>[4x]MTTLTRADWEARAKDLKIEGRA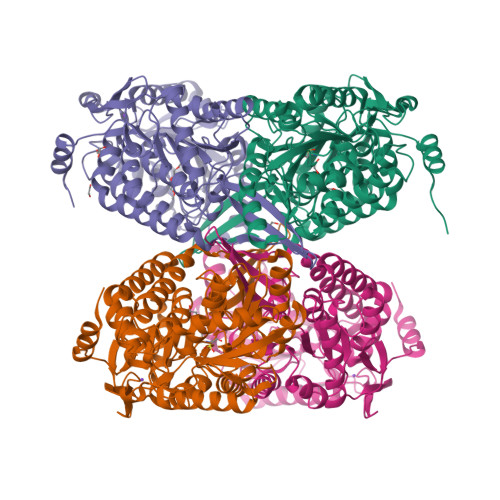FVNGEYSNAASGETFDCLSPVDGRFLAKVASCDLADAEQAVKVARNAFDSGAWSRLAPAKRKQTMIRFADLLLENAEELALLETLDMGKPISDSLHIDVASAANSLRWSAEAIDKIYDEVAATPHAELGLVTREPVGVVAAIVPWNFPLLMSCWKLGPALATGNSVILKPSEKSPLTAIRIAQLAVEAGIPKGVFNVLPGYGHTVGKALALHMDVDTLVFTGSTKIAKQLMVYAGESNMKRVWLEAGGKSPNIVFADAPDLKAAAEAAAGAIAFNQGEVCTAGSRLLVERSIKDKFLPLVIEALKGWKPGNPLDPETNVGALVDTQQMNTVLSYIEAGHNDGAKLVAGGKRTLEETGGTYVEPTIFDGVTNAMKIAREEIFGPVLSVIEFEDAEEAVRIANDTPYGLAAAVWTSNLSKAHLTAKALRAGSVWVNQYDGGDMTAPFGGFKQSGNGRDKSLHAFDKYTELKATWIKL> GPLGSSKKRKRSRWNQDTMEQKTVIPGMPTVIPPGLTREQERAYIVQLQIEDLTRKLRTGDLGIPPNPEDRSPSPEPIYNSEGKRLNTREFRT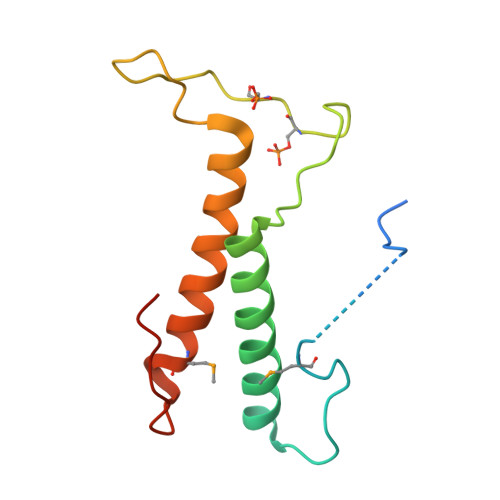RKKLEEERHNLITEMVALNPDFKPPADYKPP> MILDTDYITEDGKPVIRIFKKENGEFKIEYDRTFEPYFYALLKDDSAIEEVKKITAERHGTVVTVKRVEKVQKKFLGRPVEVWKLYFTHPQDVPAIRDKIREHPAVIDIYEYDIPFAKRYLIDKGLVPMEGDEELKMLAFAIATLYHEGEEFAEGPILMISYADEEGARVITWKNVDLPYVDVVSTEREMIKRFLRVVKEKDPDVLITYNGDNFDFAYLKKRCEKLGINFALGRDGSEPKIQRMGDRFAVEVKGRIHFDLYPVIRRTINLPTYTLEAVYEAVFGQPKEKVYAEEITTAWETGENLERVARYSMEDAKVTYELGKEFLPMEAQLSRLIGQSLWDVSRSSTGNLVEWFLLRKAYERNELAPNKPDEKELARRRQSYEGGYVKEPERGLWENIVYLDFRSLYPSIIITHNVSPDTLNREGCKEYDVAPQVGHRFCKDFPGFIPSLLGDLLEERQKIKKKMKATIDPIERKLLDYRQRAIKILANSYYGYYGYARARWYCKECAESVTAWGREYITMTIKEIEEKYGFKVIYSDTDGFFATIPGADAETVKKKAMEFLKYINAKLPGALELEYEGFYKRGFFVTKKKYAVIDEEGKITTRGLEIVRRDWSEIAKETQARVLEALLKDGDVEKAVRIVKEVTEKLSKYEVPPEKLVIHEQITRDLKDYKATGPHVAVAKRLAARGVKIRPGTVISYIVLKGSGRIGDRAIPFDEFDPTKHKYDAEYYIENQVLPAVERILRAFGYRKEDLRYQKTRQVGLSAWLKPK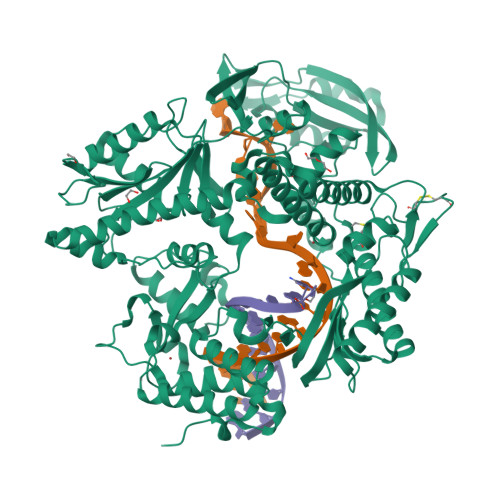GT> MESLLEKRRQLSRDIGRLKETYEALLARFPNLRFAYKDPEKNWNRNCVKGLVASLISVKDTSATTALELVAGERLYNVVVDTEVTGKKLLERGELK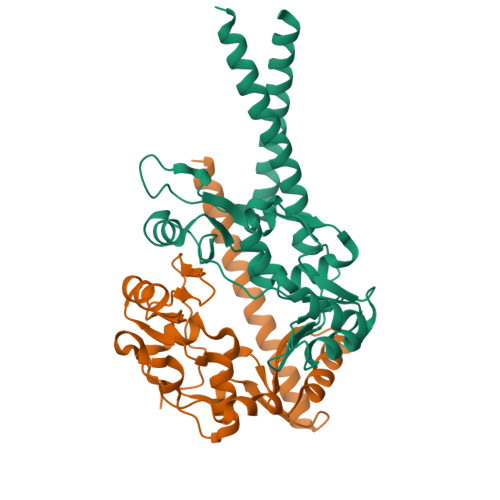RRYTIIPLNKISARCIAPETLRVAQNLVGPDNVHVALSLVEYKPELQKAMEFVFGTTFVCDNMDNAKKVAFDKRIMTRTVTLGGDVFDPHGTLSGGARSQAASILTKFQELKDVQDELRIKENELRALEEELAGLKN;> GPGTQEETNFKSLVHDLFQKVEEAKSSLAMNRSRGKVLDAIIQEKKSGRIPGIYGRLGDLGAIDEKYDVAISSCCHALDYIVVDSIDIAQECVNFLKRQNIGVATFIGLDKMAVWAKKMTEIQTPENTPRLFDLVKVKDEKIRQAFYFALRDTLVADNLDQATRVAYQKDRRWRVVTLQGQIIEQSGTMTGGGSKVMKGRMGSSLVIEISEEEVNKMESQLQNDSKKAMQIQEQKVQLEERVVKLRH> MDLTSKVNRLLAEFAGRIGLPSLSLDEEGMASLLFDEQVGVTLLLLAERERLLLEADVVGIDVLGEGIFRQLASFNRHWHRFDLHFGFDELTGKVQLYAQILAAQLTLECFEATLANLLDHAEFWQRLLPC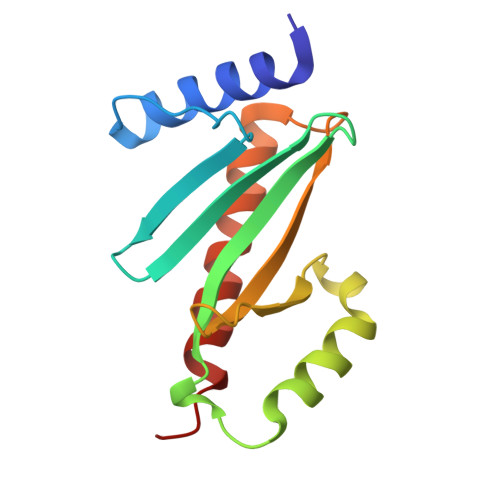AS(1~{S},3~{S},4~{S},5~{R})-3-(aminomethyl)-3,4,5-tris(hydroxyl)cyclohexane-1-carboxylic acid | C8 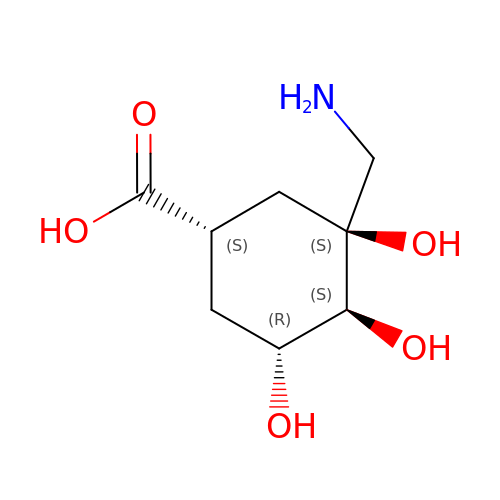H15 N O5 | YNLZKDMNCIPLRS-GCJQMDKQSA-N>[2x]GGENTPQPTDGRVALEATSGIRMNTRAYDKTWEAGDAIGIYMLNGDATDGNG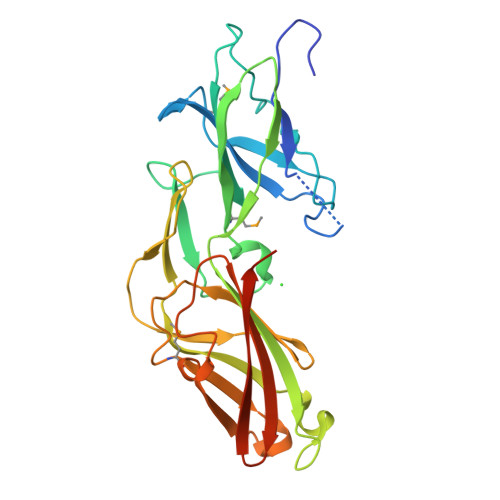NRKYTTAQTAENGSFTAAEGQTIYFPVDASQRDFVAYYPYRETLADGNVYTVDVSVQTPQKDIDLMGAAKVEGKDKTDPKVAFVFTHKLVKLDITIKADGTSLTDADLAGTTVSISNQQTAATYNVVTGGDATVTTGTTKEIVLHTDGLKAEGIVLPAASTAGMALTFTVPGLEGQAFHWDVNSAAQSKAFVAGSKYLYTITISKAGVEVSSKVEDWTPGNGGGETGNAE> MHHHHHHTLGDQGGQGQEPPPEPRITLKVGGQPVTFLVDTGAQHSVLTQNPGPLSDKSAWVQGATGGKRYRWTTDRKVHLATGKVTHSFLHVPDCPYPLLG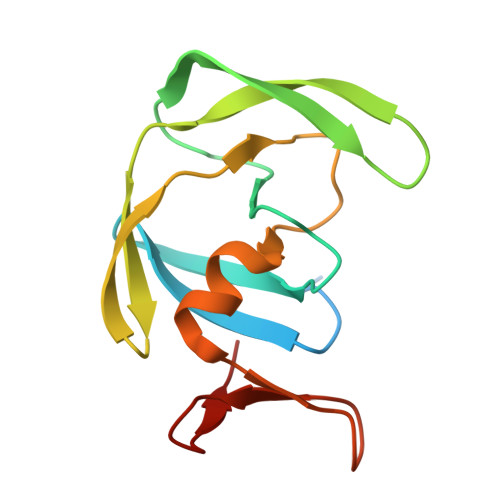RDLLTKLKAQIHFEGSGAQVVGPMGQPLQVL> MGTVSSRRSWWPLPLLLLLLLLLGPAGARAQEDEDGDYEELVLALRSEEDGLAEAPEHGTTATFHRCAKDPWRLPGTYVVVLKEETHLSQSERTARRLQAQAARRGYLTKILHVFHGLLPGFLVKMSGDLLELALKLPHVDYIEEDSSVFAQ;> SIPWNLERITPPRYRADEYQPPDGGSLVEVYLLDTSIQSDHREIEGRVMVTDFENVPEEDGTRFHRQASKCDSHGTHLAGVVSGRDAGVAKGASMRSLRVLNCQGKGTVSGTLIGLEFIRKSQLVQPVGPLVVLLPLAGGYSRVLNAACQRLARAGVVLVTAAGNFRDDACLYSPASAPEVITVGATNAQ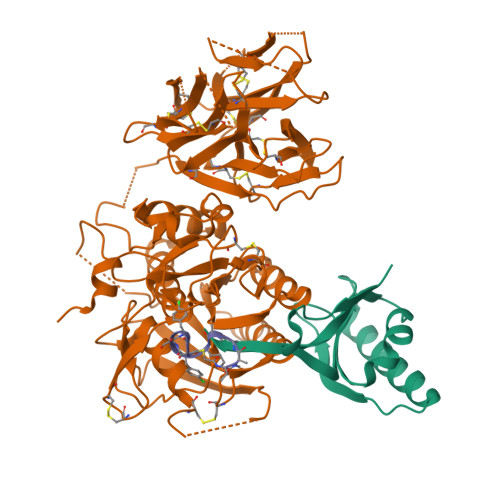DQPVTLGTLGTNFGRCVDLFAPGEDIIGASSDCSTCFVSQSGTSQAAAHVAGIAAMMLSAEPELTLAELRQRLIHFSAKDVINEAWFPEDQRVLTPNLVAALPPSTHGAGWQLFCRTVWSAHSGPTRMATAIARCAPDEELLSCSSFSRSGKRRGERMEAQGGKLVCRAHNAFGGEGVYAIARCCLLPQANCSVHTAPPAEASMGTRVHCHQQGHVLTGCSSHWEVEDLGTHKPPVLRPRGQPNQCVGHREASIHASCCHAPGLECKVKEHGIPAPQEQVTVACEEGWTLTGCSALPGTSHVLGAYAVDNTCVVRSRDVSTTGSTSEEAVTAVAICCRSRHLAQASQELQ;> XTAAALFSFAX> MAQDINADDQLKQLSALEGANGYVIFNESGIPLKRHEKSISHEKAVHIAALVSDLWNVSKK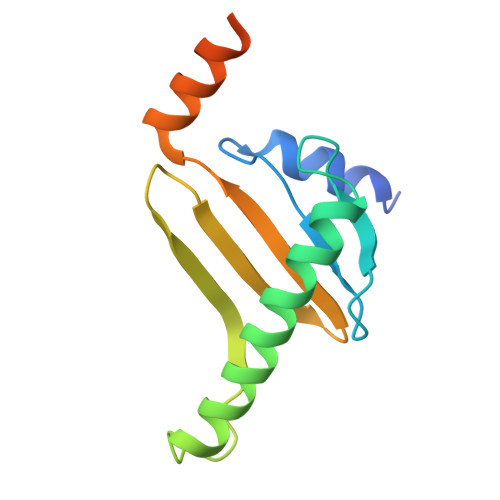VIQRDLKTPENDIEVIRLRTKHSYEYIITQSGDFTMLAIQLCGKAIEEAKKAAAAAAAAAVVQEENKEKEKK>[6x]HMHKDLHSIIDALDTAGRLIRVRSQVKAEHELAGIAAKYEGCDKAVLFENVDGNDIPVLMGLYWSRDLLGSLYGVDAVDMPRFITSKISHWKSEPTAHQLIAREHAPVMAHSPRVDLLSLPIPVHAQKDGGAYVDAGVVIAADPDTGVLNTSIQRFMVENENTLHVNIDAGRHLGAYLAKAKAK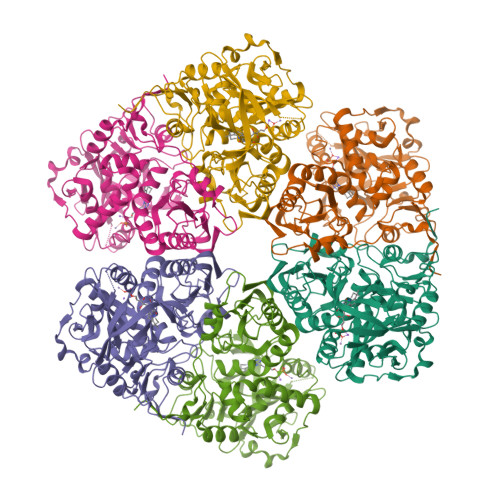GEPLSFSLNIGVHPGVHFAAATPSEVAPLDVDELGIAAEFQDGPVRIVQGDDPRVTVLADAMISLECQMYADDLADEGPFAEVTGYYAERAPRPRVTVTAVHLQRNPVFHSILSGQEVFNSVGLLGESALFDQVSKQVPGILEVALTDGGCGFYHAVVQLKQVRAGWSKQAILATFAAFPPLKMVTIVDEDVDLRNPRDVEWAMATRLDPERGILRIDDTFGHGLNPSFPDYFGSKVGFDATRSFPFEEKHERITYQDVDLSRFEIVEGHTAGGQHE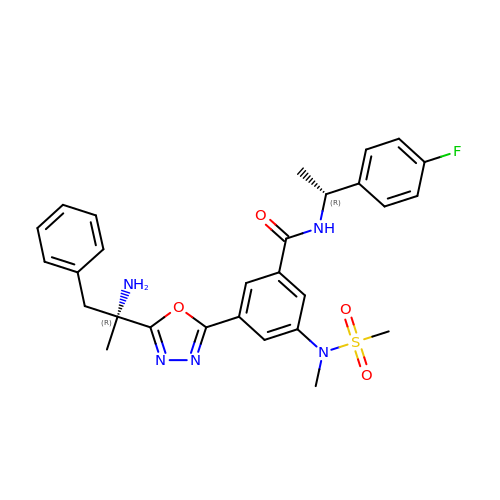3-{5-[(1R)-1-AMINO-1-METHYL-2-PHENYLETHYL]-1,3,4-OXADIAZOL-2-YL}-N-[(1R)-1-(4-FLUOROPHENYL)ETHYL]-5-[METHYL(METHYLSULFONYL)AMINO]BENZAMIDE | C28 H30 F N5 O4 S | QEJSJQVKMSAHHX-KWMCUTETSA-N>[2x]MSLAQIKSLFATRLYHAPLSEHGPALDPAEFAASCYSIAEDDDAGQEWCEREGYPGYTSYASLTDLPWRFPIFADLVKSLDAHVAAFAEDLEFE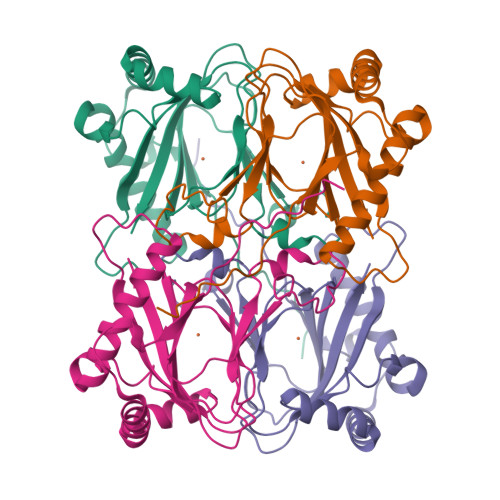LDGKALRLEDIWINILPEGGVHGSHIHPHSVISGTTYVAMPEGTSALKLEDPRLPFMMAAPTRRKGAREELRTFRSVAPKVGDVLLWESWLRHEVPMNMAEEDRISVSFNYAWGEGHHHHHH> MKIVSWNVNGIRAALKKNLIDFIENNMFEVIMFQETKGDIVPLDFIMMGYEVISFPAKRKGYSGVMTLTKIKPINVIKGLQIKEFDDEGRTVTLELKDFYVINAAFPRAGDNLERLDFKLKFNNEIENFVLKLRRAKPVILCGDFNIAHQNIDGAFSDPTIPGLTPQERSWFSHFLSLGFIDTFRYLHPNVRKYSWWSYMGKAREKNLGLRL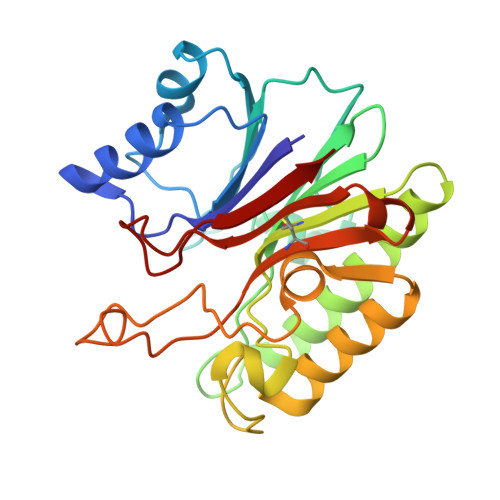DYCIVSEELKDRIKMADILIDIQGSDHAPIILELT>SNADASQFPQLTKEVGKEEAKVVMRTSQGDITLKLFPKYAPLAVENFLTHAKKGYYDNLTFHRVINDFMIQSGDPKGDGTGGESIWKGKDPKKDAGNGFVNEISPFLYHIRGALAMANAGANTNGSQFYINQNKKNQSKGLSSTNYPKPIISAYEHGGNPSLDGGYTVFGQVIDGMDVVDKIAATSINQNDKPEQDITITSIDIVKDYRFKN[2x]

Here, we solved the protein structures of two secreted parvulin and two secreted cyclophilin-like peptidyl-prolyl isomerase (PPIase) ATP-independent chaperones found in gram-positive streptococcal species. Two types of ATP-independent extracellular PPIases exist in pathogenic streptococci: the parvulin and cyclophilin families. Unlike cytoplasmic PPIases, extracellular PPIases have canonical secretion signal peptides that allow for their translocation across the cell membrane via the Sec pathway. These chaperones are lipidated to the outer leaflet of the membrane and function in the space between the bacterial membrane and cell wall.

We then solved the crystal structures of SlrA homologs from S. pneumoniae (SpnSlrA) and S. pyogenes (SpyPpiA) to 1.88 Å and 1.28 Å resolution, respectively, using single-wavelength anomalous diffraction (SAD) data from selenomethionine derivatized crystals. Although the expression construct encodes residues 21–268, three residues of the purification tag and 39 N-terminal residues were disordered in the crystal; thus, only residues 60–268 could be resolved. Superimposition of chains A from the SpnSlrA and SpyPpiA structures confirms that their structures are homologous and share good alignment with an r.m.s.d. of 2.08 Å. The SpnSlrA and SpyPpiA proteins have a canonical cyclophilin fold comprised of eight antiparallel β-strands (SpnSlrA: β1, 72–81; β2, 82–90; β3, 112–120; β4, 121–127; β5, 166–173; β6, 181–188; β7, 221–227; β8, 250–260) that form a β-barrel with two α-helices (SpnSlrA: α1,95–108; α2, 230–240) located at the top and the bottom of the barrel. Both structures also contain extra secondary structural elements adjacent to the β-barrel composed of residues 189–212 (η2, 193–195; η3, 203–211; η4, 215–217). SpnSlrA putative active site residues Phe184 and His221 are identical to hCypA residues but are substituted by Tyr in SpyPpiA. Thus, we sought to determine whether these substitutions still allow for SpyPpiA PPiase activity. SpnSlrA, SpyPpiA, and hCypA all catalyzed the cis-to-trans isomerization of the N-succinyl-Ala-Ala-Pro-Phe-p-nitroanilide substrate. However, we observed ~20% decrease in PPIase activity of SpnSlrA and SpyPpiA compared to hCpyA. These data indicate that Tyr substitutions at key putative active site positions allow for PPIase activity in, at least, one streptococcal cyclophilin. Using affinity isothermal titration calorimetry (ITC), we determined that SpnSlrA and SpyPpiA bind to CsA with a dissociation constants (Kd) of 122.4 ± 41.4 nM and 365.7 ± 102.1 nM, respectively.> 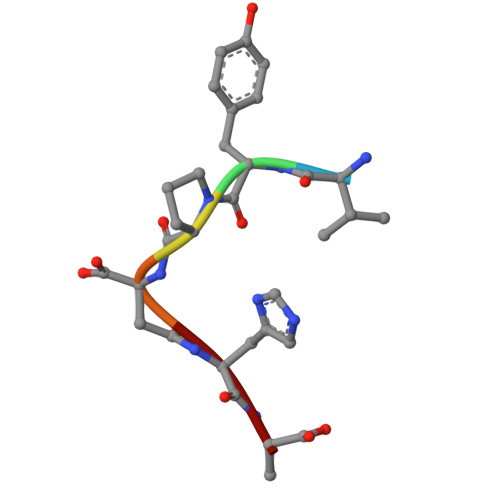VYPDHA>[4x]MLARKSIIPEEYVLARIAAENLRKPRIRDRLPKARFIAKSGACNLAHKNIREQGRFLQDIFTTLVDLKWRHTLVIFTMSFLCSWLLFAIMWWLVAFAHGDIYAYMEKGITEKSGLESAVCVTNVRSFTSAFLFSIEVQVTIGFGGRMMTEECPLAITVLILQNIVGLIINAVMLGCIFMKTAQAHRRAETLIFSRHAVIAVRNGKLCFMFRVGDLRKSMIISASVRIQVVKKTTTPEGEVVPIHQQDIPVDNPIESNNIFLVAPLIICHVIDKRSPLYDISATDLVNQDLEVIVILEGVVETTGITTQARTSYIAEEIQWGHRFVSIVTEEEGVYSVDYSKFGNTVRVAAPRCSARELDEKPSILIQTLQKSELSHQNSLRKRNSMRRNNSMRRSNSIRRNNSSLMVPKVQFMTPEGNQCPSES;> MSLSFCGNNISSYNIYHGVLQNPCFVDALNLVPHVFLLFITFPILFIGWGSQSSKVQIHHNTWLHFPGHNLRWILTFALLFVHVCEIAEGIVSDSQRASRHLHLFMPAVMGFVATTTSIVYYHNIETSNFPKLLLALFLYWVMAFITKTIKLVKYWQLGWGMSDLRFCITGVMVILNGLLMAVEINVIRVRRYVFFMNPQKVKPPEDLQDLGVRFLQPFVNLLSKATYWWMNTLIISAHRKPIDLKAIGKLPIAMRAVTNYVCLKEAYEEQKKKAADHPNRTPSIWLAMYRAFGRPILLSSTFRYLADLLGFAGPLCISGIVQRVNEPKNNTTRFSETLSSKEFLENAHVLAVLLFLALILQRTFLQASYYVTIETGINLRGALLAMIYNKILRLSTSNLSMGEMTLGQINNLVAIETNQLMWFLFLCPNLWAMPVQIIMGVILLYNLLGSSALVGAAVIVLLAPIQYFIATKLAEAQKSTLDYSTERLKKTNEILKGIKLLKLYAWEHIFCKSVEETRMK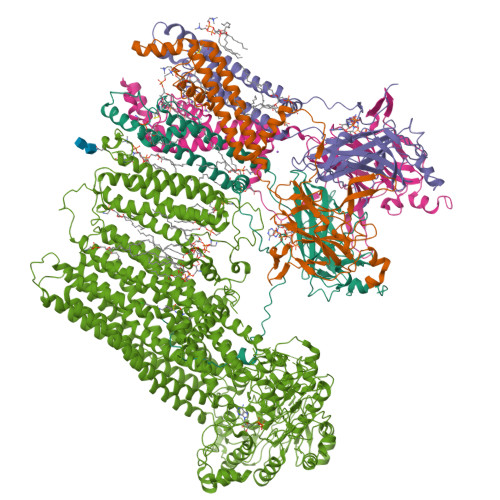ELSSLKTFALYTSLSIFMNAAIPIAAVLATFVTHAYASGNNLKPAEAFASLSLFHILVTPLFLLSTVVRFAVKAIISVQKLNEFLLSDEIGEDSWRTGEGTLPFESCKKHTGVQSKPINRKQPGRYHLDNYEQARRLRPAETEDVAIKVTNGYFSWGSGLATLSNIDIRIPTGQLTMIVGQVGCGKSSLLLAILGEMQTLEGKVYWNNVNESEPSFEATRSRSRYSVAYAAQKPWLLNATVEENITFGSSFNRQRYKAVTDACSLQPDIDLLPFGDQTEIGERGINLSGGQRQRICVARALYQNTNIVFLDDPFSALDIHLSDHLMQEGILKFLQDDKRTVVLVTHKLQYLTHADWIIAMKDGSVLREGTLKDIQTKDVELYEHWKTLMNRQDQELEKDMEADQTTLERKTLRRAMYSREAKAQMEDEDEEEEEEEDEDDNMSTVMRLRTKMPWKTCWWYLTSGGFFLLFLMIFSKLLKHSVIVAIDYWLATWTSEYSINDPGKADQTFYVAGFSILCGAGIFLCLVTSLTVEWMGLTAAKNLHHNLLNKIILGPIRFFDTTPLGLILNRFSADTNIIDQHIPPTLESLTRSTLLCLSAIGMISYATPVFLIALAPLGVAFYFIQKYFRVASKDLQELDDSTQLPLLCHFSETAEGLTTIRAFRHETRFKQRMLELTDTNNIAYLFLSAANRWLEVRTDYLGACIVLTASIASISGSSNSGLVGLGLLYALTITNYLNWVVRNLADLEVQMGAVKKVNSFLTMESENYEGTMDPSQVPEHWPQEGEIKIHDLCVRYENNLKPVLKHVKAYIKPGQKVGICGRTGSGKSSLSLAFFRMVDIFDGKIVIDGIDISKLPLHTLRSRLSIILQDPILFSGSIRFNLDPECKCTDDRLWEALEIAQLKNMVKSLPGGLDATVTEGGENFSVGQRQLFCLARAFVRKSSILIMDEATASIDMATENILQKVVMTAFADRTVVTIAHRVHTILTADLVIVMKRGNILEYDTPESLLAQEDGVFASFVRADM> SPSAEACGYSDRVLQLKLGNSSIVTQEAANICCAYGEWPTYLPDNEAVAIDKPTQPETSTDRFYTLKSKKWESNSTGWWWKLPDALNQIGMFGQNVQYHYLYRSGFLCHVQCNATKFHQGTLLIVAIPEHQIGKKGTGTSASFAEVMKGAEGGVFEQPYLLDDGTSLACALVYPHQWI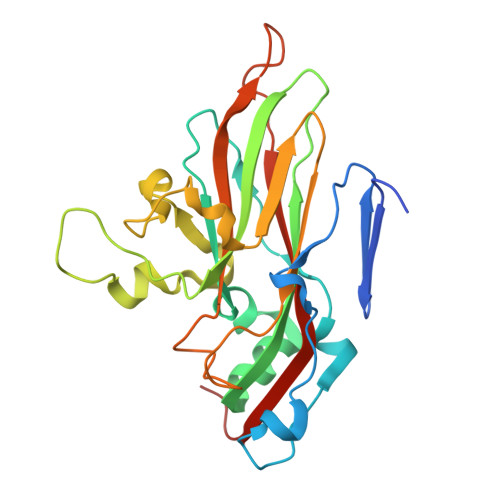NLRTNNSATIVLPWMNSAPMDFALRHNNWTLAVIPVCPLAGGTGNTNTYVPITISIAPMCAEYNGLRNAITQ> MKTVTVKNLIIGEGMPKIIVSLMGRDINSVKAEALAYREATFDILEWRVDHFMDIASTQSVLTAARVIRDAMPDIPLLFTFRSAKEGGEQTITTQHYLTLNRAAIDSGLVDMIDLELFTGDADVKATVDYAHAHNVYVVMSNHDFHQTPSAEEMVLRLRKMQALGADIPKIAVMPQSKHDVLTLLTATLEMQQHYADRPVITMSMAKEGVISRLAGEVFGSAATFGAVKQASAPGQIAVNDLRSVLMILHNA

Several studies have identified the enzyme type I dehydroquinase (DHQ1, 3-dehydroquinate dehydratase, EC 4.2.1.10) as a promising target for anti-virulence drug development. DHQ1 catalyzes the reversible dehydratation of 3-dehydroquinic acid (1) to 3-dehydroshikimic acid (2), which is the third step in the shikimic acid pathway. It follows a covalent catalysis mechanism with the formation of transient Schiff base species´ between the ketone moiety of the substrate and the ɛ-amino group of a catalytic lysine residue (K160/K170 in Sa-DHQ1 and St-DHQ1, respectively), which are finally hydrolyzed to regenerate the enzyme. An essential histidine residue (H133/H143 in Sa-DHQ1 and St-DHQ1, respectively), is also involved in the formation/hydrolysis of the Schiff base intermediates.

In addition, the reactivity of C3 in the quinate scaffold was also explored by introduction of an oxirane moiety with an S,S configuration at the C2-C3 bond (compound 8) to compare the geometry requirements of the C3 position towards nucleophilic attack. Despite having a reactive electrophilic warhead, compound 8 proved to be a reversible competitive inhibitor of the enzyme and was very stable in the enzyme active site, as evidenced by resolution of the crystal structure of the Salmonella typhi DHQ1 enzyme in complex with 8 at 1.55 Å. The crystal structure of St-DHQ1 in complex with epoxide 8 crystallized with one molecule in the asymmetric unit and was solved at a resolution of 1.55 Å. The calculated maps revealed clear high electron density for the ligand molecule 8, which binds to the active site via a salt bridge between its C1 carboxylate group and the guanidinium group of the conserved R213, along with a network of attractive hydrogen-bonding interactions with several side-chain residues. The enzyme structure shows that the introduction of a three-membered ring at the C2 and C3 positions of the cyclohexane ring in the ligand causes a twist in the overall chair conformation and, as a result, the strength of the contacts of the C5 hydroxyl group, as well as the accessibility to the C3 carbon by the ɛ-amino group of K170, are altered. Thus, the hydrogen bond between the C5 hydroxyl group in 8 and the carboxylate group of E46 is 0.3 Å longer than in the St-DHQ1/6 adduct, while the interaction with residue R48 is shortened by 0.2 Å (Figures 4C vs 3C). More importantly, the CH group in the C3 position in 8 is twisted towards the bottom of the active site, thus hindering the reaction with the ɛ-amino group of K170, and the side chain of H143 is positioned close enough to the oxirane moiety in 8 (3.0 Å) for potential activation (Lewis acid). In addition, residue K170 shows a bent arrangement, and its ɛ-amino group is located pointing towards the carboxylate group of D114 (3.1 Å) and the structural water molecule (3.1 Å). The unsuitable orientation of the oxirane functional group within the cyclic compound might justify the lack of covalent modification observed experimentally.>SALEGKIAKLEHAEACAATASGMGA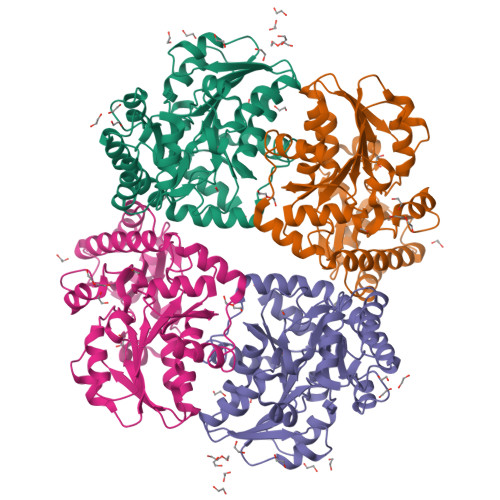IAASVWTFLKAGDHLISDDCLYGCTHALFEHQLRKFGVEVDFIDMAVPGNIEKHLKPNTRIVYFETPANPTLKVIDIEDAVKQARKQKDILVIVDNTFASPILTNPLDLGVDIVVHSATKYINGHTDVVAGLVCSRADIIAKVKSQGIKDITGAIISPHDAWLITRGTLTLDMRVKRAAENAQKVAEFLHEHKAVKKVYYPGLPDHPGHEIAKKQMKMFGSMIAFDVDGLEKAKKVLDNCHVVSLAVSLGGPESLIQHPASMTHAGVPKEEREAAGLTDNLIRLSVGCENVQDIIDDLKQALDLVL[2x]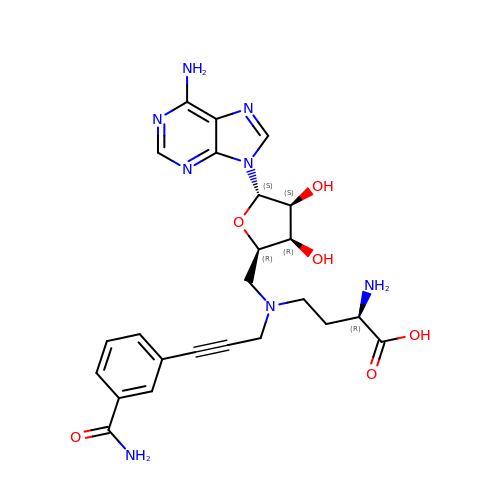9-(5-{[(3R)-3-amino-3-carboxypropyl][3-(3-carbamoylphenyl)prop-2-yn-1-yl]amino}-5-deoxy-alpha-D-lyxofuranosyl)-9H-purin-6-amine | C24 H28 N8 O6 | BWPXKNJHQXYKGO-VUZQMMKOSA-N URIDINE-DIPHOSPHATE-2(N-ACETYLGLUCOSAMINYL) 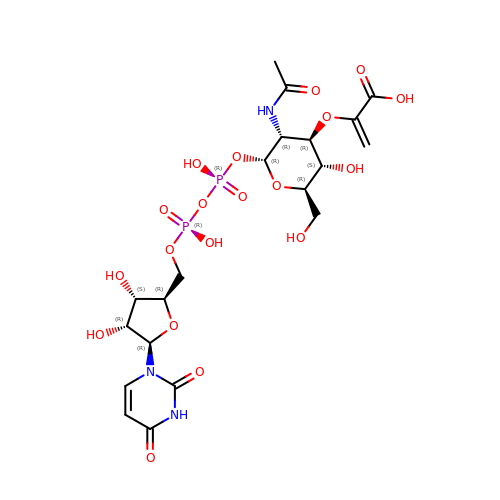BUTYRIC ACID | C20 H29 N3 O19 P2 | BEGZZYPUNCJHKP-DBYWSUQTSA-N> MANGYTYEDYQDTAKWLLSHTEQRPQVAVICGSGLGGLVNKLTQAQTFDYSEIPNFPESTVPGHAGRLVFGILNGRACVMMQGRFH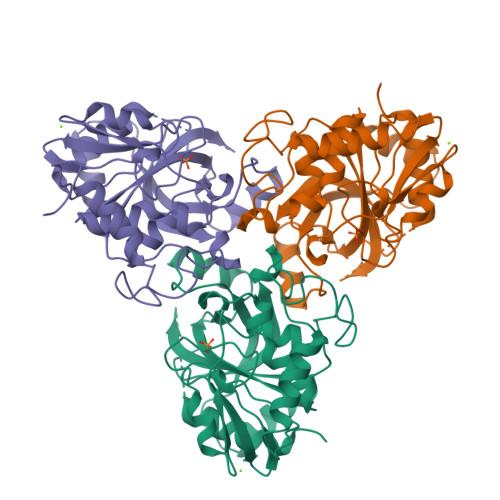MYEGYPFWKVTFPVRVFRLLGVETLVVTNAAGGLNPNFEVGDIMLIRDHINLPGFSGENPLRGPNEERFGVRFPAMSDAYDRDMRQKAHSTWKQMGEQRELQEGTYVMLGGPNFETVAECRLLRNLGADAVGMSTVPEVIVARHCGLRVFGFSLITNKVIMDTESQGKANHEEVLEAGKQAAQKLEQFVSLLMASIPVSGHTG>[2x]MRWENLFVSGVAAWLPPLSTAQDAVMAGLLDPARSKLRGIESVTVASDAEEDAPPRMAARAARAALGRGDVDPADVSLVLHSSLWFQGIDLWPAA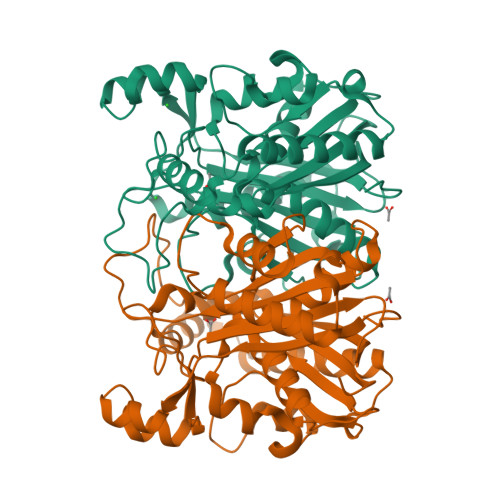SYVAHEAVGRHVPAFGLAQRCNGGMGAIELAGAYLGSGIGAGHAALLTTGDRFAGPRIDRWNSVDVTMYGDGAAALVLSTRDGFARVLSTATGVDNSLEILARGDEPFAPHPVEPSPVADLGTRTVRGAELADLPDLTHRYIDLLVAAKTQALEDAGTAIEDIAHAVIPVSRRGTGHELHDLLGLPDERTSWAYGRTTGHVGAGDQYAGLAHLVENALVQPGDRVLLFGGGAGYTCTAAVVEILRMPAQCMRGSRSHHHHHH>QNWATFQQKHIINTPIINCNTIMDNNIYIVGGQCKRVNTFIISSATTVKAICTGVINMNVLSTTRFQLNTCTRTSITPRPCPYSSR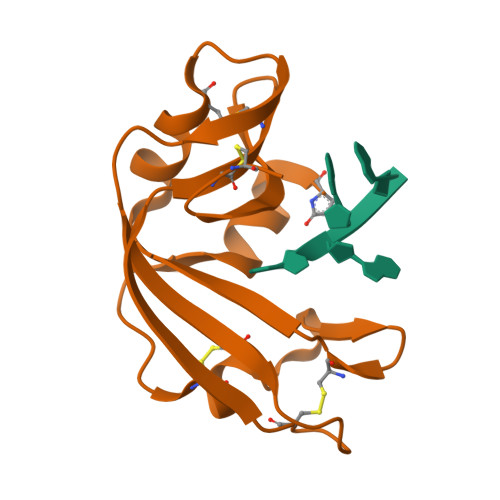TETNYICVKCENQYPVHFAGIGRCP[2x]> ATPKQGPRMLGAPEEADANEEGVRRALDFAV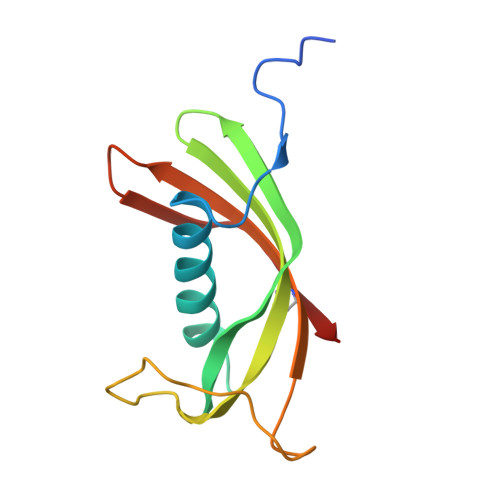SEYNKGSNDAYHSRAIQVVRARKQLVAGVNYFLDVEMGRTTCTKSQTNLTDCPFHDQPHLMRKALCSFQIYSVPWKGTHSLTKFSCKNA> MLDDAHSLRCNLTIKAPTPADPLWYEAKCLVDEILILHLSNINKTMTSGDPGETANATEVGECLTQPVNDLCQKLRDKVSNTKVDTHKTNGYPHLQVTMIYPQSQGQTPSATWEFNISDSYFFTFYTENMSWRSANDESGVIMNKWNDDGDLVQRLKYFIPECRQKIDEFLKQSK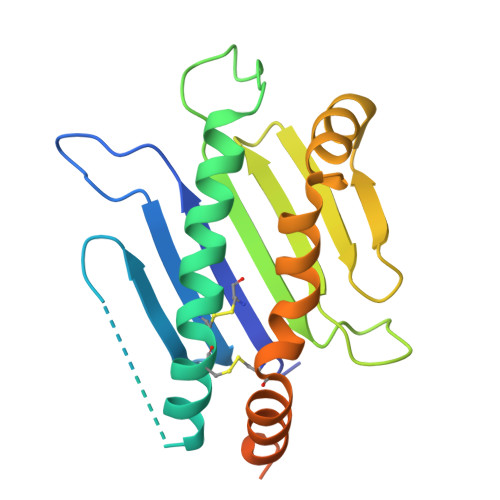EKPRSTSRSPSITQLTSTSPLPPPSHSTSK>[3x]MLEGKFEEAALLKKVVEAIKDCVKKCNFNCSEHGITVQAVDDSRVLLVSLLIGQTSFSEYRCDRDVTLGIDLESFSKIIKSANNEDFLTLLAEDSPDQIMAILEEKQKEKISEYSLKLMDIDSEFLQIDDMEYDAVVNMPSSDFAKLVRDLKNLSESLRVVVTKDSVKFTSEGDSGSGSVILKPYTNLKNERESVTISLDDPVDLTFGLKYLNDIVKAATLSDVITIKL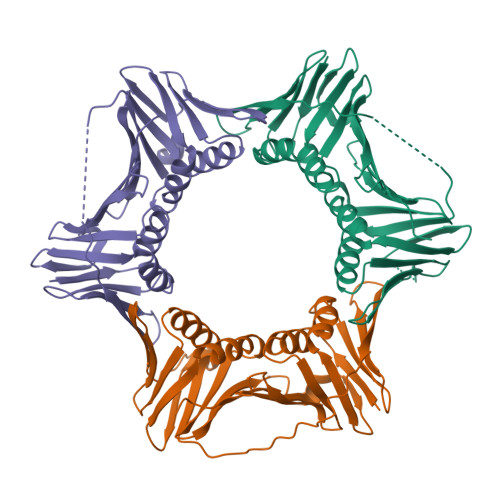ADKTPALFEFKMQSGGYLRFYLAPKFDDDELEHHHHHH> MSDTMVVNGSGGVPAFLFSGSTLSSYRPNFEANSITIALPHYVNLPGRSNFKLMYIMGFPIDTEMEKDSEYSNKIRQESKISKTEGTVCYEQKITVETGQEKDGVKVYRVMVLEGTIAESIEHLDKKENEDILNNNRNRIVLADNTVINFDNISQLKEFLRRSVNIVDHDIFSSNGFEGFNPTSHFPSNPSSDYFNSTGVTFGSGVDLGQRSKQDLLNDGVPQYIADRLDGYYMLRGKEAYDKVRTAPLTLSDNEAHLLSNIYIDKFSHKIEGLFNDANIGLRFCDLPLRTRTALVSIGYQKGFKLSRTAPTVWNKVIAKDWNGLVNAFNNIVDGMSDRRKREGALVQKDIDSGLLK;> MSDTMVVNGSGGVPAFLFSGSTLSSYRPNFEANSITIALPHYVDLPGRSNFKLMYIMGFPIDTEMEKDSEYSNKIRQESKISKTEGTVCYEQKITVETGQEKDGVKVYRVMVLEGTIAESIEHLDKKENEDILNNNRNRIVLADNTVINFDNISQLKEFLRRSVNIVDHDIFSSNGFEGFNPTSHFPSNPSSDYFNSTGVTFGSGVDLGQRSKQDLLNDGVPQYIADRLDGYYMLRGKEAYDKVRTAPLTLSDNEAHLLSNIY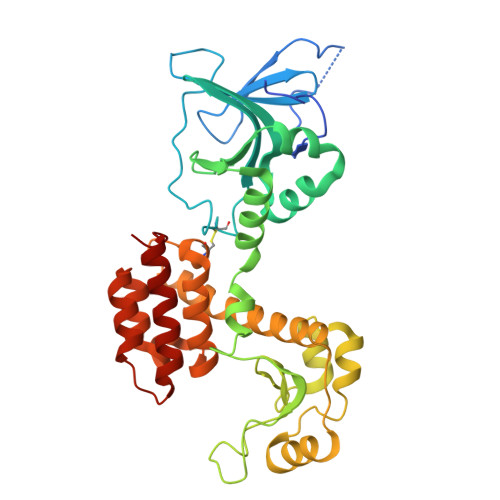IDKFSHKIEGLFNDANIGLRFCDLPLRTRTALVSIGYQKGFKLSRTAPTVWNKVIAKDWNGLVNAFNNIVDGMSDRRKREGALVQKDIDSGLLK> MAGGAFVSEGGGGGRSYEGGVTAFVIMTCIVAAMGGLLFGYDLGISGGVTSMEEFLTKFFPQVESQMKKAKHDTAYCKFDNQMLQLFTSSLYLAALVASFMASVI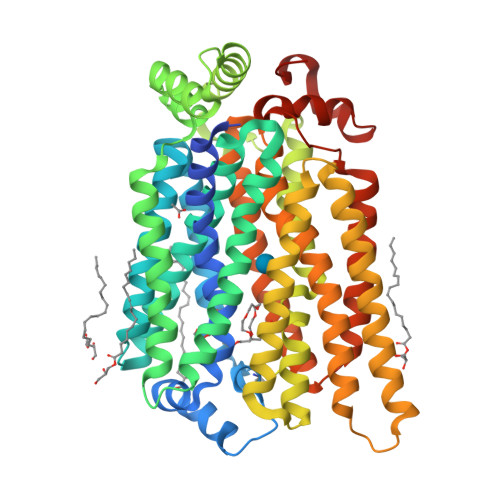TRKHGRKVSMFIGGLAFLIGALFNAFAVNVSMLIIGRLLLGVGVGFANQSTPVYLSEMAPAKIRGALNIGFQMAITIGILVANLINYGTSKMAQHGWRVSLGLAAVPAVVMVIGSFILPDTPNSMLERGKNEEAKQMLKKIRGADNVDHEFQDLIDAVEAAKKVENPWKNIMESKYRPALIFCSAIPFFQQITGINVIMFYAPVLFKTLGFGDDAALMSAVITGVVNMLSTFVSIYAVDRYGRRLLFLEGGIQMFICQLLVGSFIGARFGTSGTGTLTPATADWILAFICVYVAGFAWSWGPLGWLVPSEICPLEIRPAGQAINVSVNMFFTFLIGQFFLTMLCHMKFGLFYFFASMVAIMTVFIYFLLPETKGVPIEEMGRVWKQHWFWKKYIPEDAIIGGHDDNNTN>[4x]GHHHHH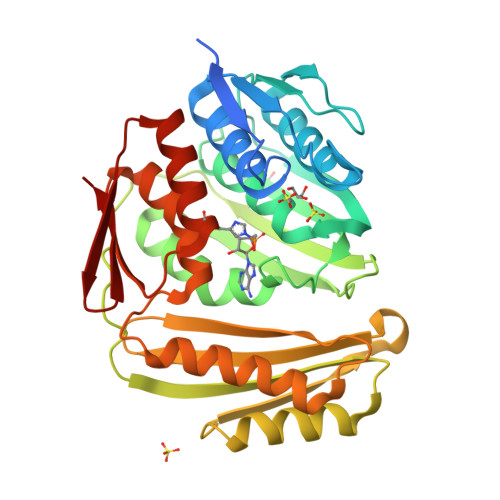HHHHHSSGHIEGRHMKRMIALDGAQGEGGGQILRSALSLSMITGQPFTITSIRAGRAKPGLLRQHLTAVKAATEICGATVEGAELGSQRLLFRPGTVRGGDYRFAIGSAGSCTLVLQTVLPALWFADGPSRVEVSGGTDNPSAPPADFIRRVLEPLLAKIGIHQQTTLLRHGFYPAGGGVVATEVSPVASFNTLQLGERGNIVQMRGEVLLAGVPRHVAEREIATLAGSFSLHEQNIHNLPRDQGPGNTVSLEVESENITERFFVVGEKRVSAEVVAAQLVKEVKRYLASTAAVGEYLADQLVLPMALAGAGEFTVAHPSCHLLTNIAVVERFLPVRFSLIETDGVTRVSIE>YLQLLILLPSSPFMVVEPHTLNYQTVTFTTKNATKTSYTQFIEALRAQLASGEEPHGIPVMRERSTVPDSKRFILVELSNWAADSPVTLAVDVTNAYVVAYRTGSQSFFLREDNPDPAIENLLPDTKRYTFPFSGSYTDLERVAGERREEILLGMDPLENAISALWISNLNQQRALARSLIVVIQMVAEAVRFRFIEYRVRESISRAEMFRPDPAMLSLENKWSALSNAVQQSNQGGVFSSPVELRSISNKPVYVGSVSDRVISGLAIMLFICRSTDRASSDQFIDHLLMIRPILADVADVATDADNDDTCADPEPTVRISGRNGLCVRVRDGKYNNGNPI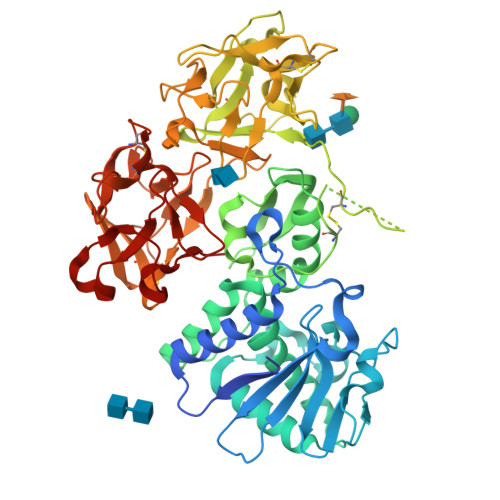QLWPCKQNSDVNQLWTLRRDGTIRSNGKCLTTNGYSAGDYVMIYDCRTPVTAASIWQFWANGTIINPQSALVLSAESGNPRTTLTVQADIYASRQGWLAGNNTEPFVTSIVGFNDLCMQANGDAMWVVECESSKAEQKWALYPDGSIRPHQDRDRCLTSTDNHSQGSIIIISSCSPGSEGQRWVFMNDGTILNLKNGLVMDVKGSDPSLHQIIIWPATGKPNQKWLPLL[2x]> MIIPALDLIGGTVVRVVRLHQGDYARQRDYGNDPLPRLQDYAAQGAGVLHL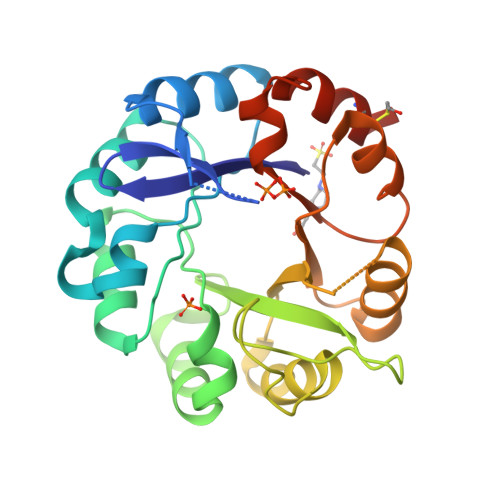VDLTGAKDPAKRQIPLIKTLVAGVNVPVQVGGGVRTEEDVAALLKAGVARVVIGSTAVKSPDVVKGWFERFGAQALVLALDVRIDEHGTKQVAVSGWQENSGVSLEQLVETYLPVGLKHVLCTDISRDGTLAGSNVSLYEEVCARYPQIAFQSSGGIGDIDDIAALRGTGVRGVIVGRALLEGKFTVKEAIQCWQNVKGHHHHHH> GAMASRKSTASSLLLRQYRELTDPKKAIPSFHIELEDDSNIFTWNIGVMVL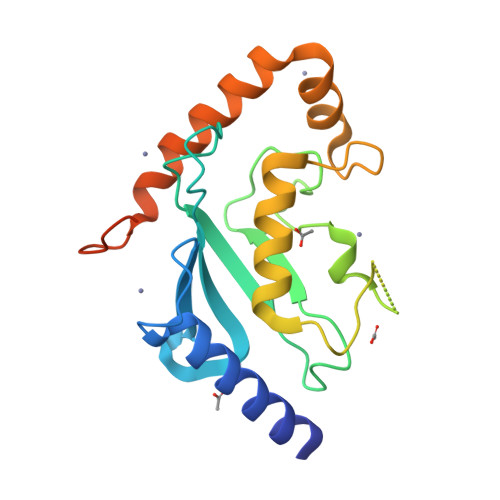NEDSIYHGGFFKAQMRFPEDFPFSPPQFRFTPAIYHPNVYRDGRLCISILHQSGDPMTDEPDAETWSPVQTVESVLISIVSLLEDPNINSPANVDAAVDYRKNPEQYKQRVKMEVERSKQDIPKGFIMPTSESAYISQSKLDEPES>[3x]ATNDDDVKKIATVALAAAYNNGQEINGFKAGETIYDIDEDGTITKKDATAADVEADDFKGLGLKKVVTN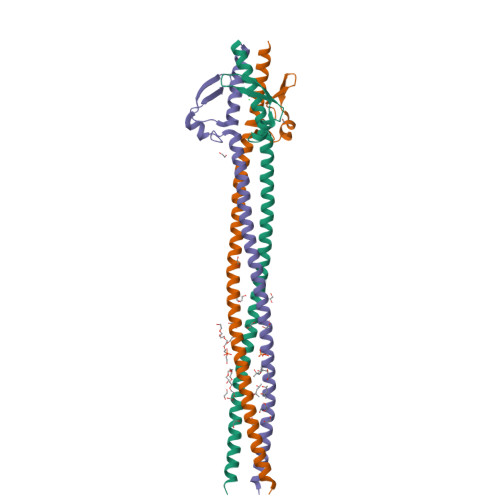LTKTVNENKQNVDAKVKAAESEIEKLTTKLADTDAALADTDAALDATTNALNKLGENITTFAEETKTNIVKIDEKLEAASKHHHHHH>[4x]GVTIAINYDYNENLWLEQQLKQKFGLKDVVVVSGNDEDEETQLAMMGLHGAQLLDRLLEPGDIVGFSWGRAVSALVENLPQAGQSRQLICVPIIGGPSGKLESRYHVNTLTYSAAAKLKGESHLADFPALLDNPLIRNGIMQSQHFKTISAYWDNL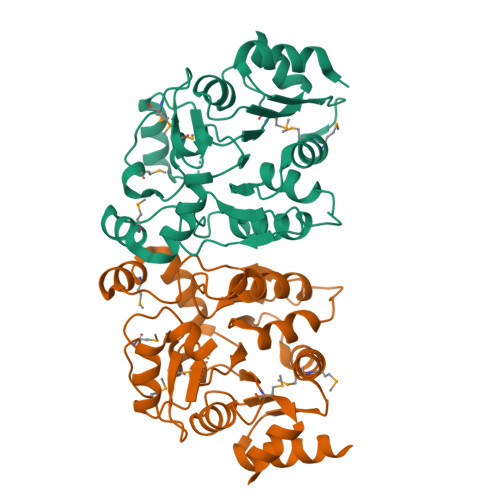DIALVGIGSPAIRDGANWHAFYGGEESDDLNARQVAGDICSRFFDIHGAMVETNMSEKTLSIEMNKLKQARYSIGIAMSEEKYSGIIGALRGKYINCLVTNSSTAELLLK>QEQVAPPKDPAAALEDHKTRTDNRYEPSLDNLAQQDVAAPGAPEGVTALSDAQYNEANKIYFERCAGCHGVLRKGATGKALTPDLTRDLGFDYLQSFITYASPAGMPNWGTSGELSAEQVDLMANYLLLDPAAPPEFGMKEMRESWKVHVAPEDRPTQQMNDWDLENLFSVTLRDAGQIALIDGSTYEIKTVL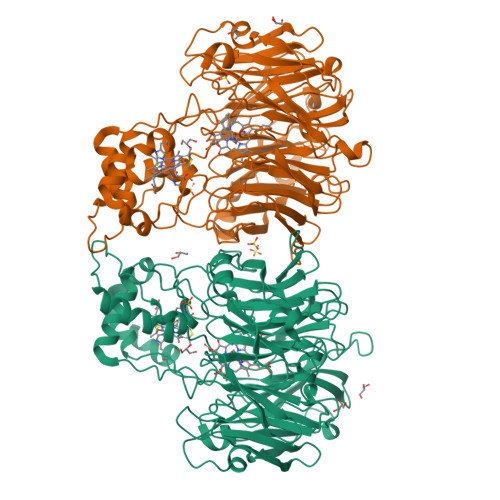DTGYAVHISRLSASGRYLFVIGRDGKVNMIDLWMKEPTTVAEIKIGSEARSIETSKMEGWEDKYAIAGAYWPPQYVIMDGETLEPKKIQSTRGMTYDEQEYHPEPRVAAILASHYRPEFIVNVKETGKILLVDYTDLNNLKTTEISAERFLHDGGLDGSHRYFITAANARNKLVVIDTKEGKLVAIEDTGGQTPHPGRGANFVHPTFGPVWATSHMGDDSVALIGTDPEGHPDNAWKILDSFPALGGGSLFIKTHPNSQYLYVDATLNPEAEISGSVAVFDIKAMTGDGSDPEFKTLPIAEWAGITEGQPRVVQGEFNKDGTEVWFSVWNGKDQESALVVVDDKTLELKHVIKDERLVTPTGKFNVYNTMTDTY[2x]In order to advance understanding of the specificity of GH149 enzymes, we herein solved X‐ray crystallographic structures of GH149 enzyme Pro_7066 in the absence of substrate and in complex with laminarihexaose (G6). We have characterized two enzymes from this family, one from the microalga Euglena gracilis, and the other a bacterial enzyme from a metagenomic library, Pro_7066. Both enzymes were shown to have substrate specificity for β‐(1 → 3)‐gluco‐oligosaccharides. The domains present within each subunit can be defined as follows: an N‐terminal β‐sandwich (residues 1‐303, yellow), a helical linker region (residues 304‐341, lilac), an (α/α)6 catalytic domain (residues 342‐1045, green) and a C‐terminal jelly roll domain (residues 1046‐1156, red).

X‐ray crystallography was used to determine the structure of Pro_7066: the substrate‐free structure was solved to 2.05 Å resolution. However, useful data could only be obtained from the G6 co‐crystallization, the structure of which was solved to 2.25 Å resolution. Both structures belong to space group P212121 and contain two subunits per ASU. The two copies of the molecule in the ASU form a biologically relevant homodimer with an interfacial area of ∼4230 Å2 were calculated by jsPISA. The formation of a homodimer in the crystal structure is consistent with the gel filtration analysis, where Pro_7066 was eluted as a dimer. The architecture of the Pro_7066 active site is highly similar to that observed for GH94 enzymes. Bicine (BCN) derived from the crystallization precipitant was bound via hydrogen bonding contacts with R470 and E951, possibly mimicking the interaction of the enzyme active site with the hydroxy groups on C3 and C6 of Glc1P donor. A sulfate molecule was observed (ice blue) occupying a similar position to the phosphate moiety of Glc1P in the PsLBP structure (magenta). Although the RMSD values suggest that these structures are not highly similar (RMSD > 1 Å), the structural elements neighboring the active site are relatively well conserved: (a) the gate (blue) described in PsLBP can be identified in Pro_7066, although in the latter it is part of a disordered loop; (b) the opposing (red) and the adjacent loops (brown), which are present in all of the three structures. In the Pro_7066 structure, Dom 2 (green) is found in proximity to the gate. The average B‐factor of Dom 2 (∼70 Å2) is higher than the average B‐factor of the protein subunit (48 Å2), suggesting Dom 2 is more dynamic compared to the rest of the subunit.

>[2x]MGSSHHHHHHSSGLVPAGSMSQSPNTLANEETTSIDKSITMDMVSMNGEMFYKIANNDAMRPFFMTIVSDSNHWMFVSSNGGLTAGRKNAEYALFPYYTDDKITESADITGSKSIFQIQYNNELIVWEPFSERFTNKFKITRNLYKNYYGNKIIFEEINEDLGLTYRYQWCSSNQFGFVRKSELSNHSKNVYEISLLDGIQNIMPYGVSSDLQSSTSNLVDAYKRSELHPKSGLGIFALSAIIVDKAEPSEALKANIAWSLGLNNPKYLVSSLQLNHFRNGKSISPEDDIKGEKGAYFLNTVMTLEANTQKEWMIIANVNQDHSDIIAITETIQNNKKIAEDINTDIELGTKRLIELNASSDALQLTADNLRDTRHFSNTLFNIMRGGIFDNNYQIEKGDFSNYIKKANKLVFDKIDLNALGEIFSLNDLNEFASKQKDVDFDRLALEYLPLKFSRRHGDPSRPWNKFSINTQSEIDGSKVLDYEGNWRDIFQNWEALAHSFPNFIDSMIHKFLNASTFDGYNPYRVTKEGFDWETIEEDDPWSYIGYWGDHQIIYLLKFLEFIEKHQPGKLHSYFESECFVYAAVPYTIKPYEEILNNPKDTIGYNHEWEKVINERKKSIGADGALLKSNDKSIYHVNFIEKILATVLAKMSNFIPEAGIWLNTQRPEWNDANNALVGNGVSMVTLYYLRRFLKFFDQLLENSTLENIKISNEMVEFYHKVRETLMENQHLLAGSISDTDRKVILDKLGNAAADYRFQIYNSGFWGKKRTHSMQGLKNFTKVSLQFIDHSIKANQRPDKLYHAYNLMSVEKNKEIAISYLSEMLEGQVAVLSSGFLSSKENLAVLDGLKNSALFREDQYSYLLYPNKELPKFLDKNTISKEAVSKSELLSLLVSKSNKQVIEKDSIGEYHFNGEFNNASNLKQALEDLSQQNEYKDLVAKESKTVEAIFEDVFNHKAFTGRSGTFYGYEGLGSIYWHMVSKLQLAVLECCLKAVEEKESEEVIGRLLEHYYEINEGIGVHKSPSLYGAFPTDAYSHTPAGKGAQQPGMTGQVKEDILSRFGELGIFVKNGCLELNPCLLRKDEFLKEAKTFDYVTVNFQHQSLELVEKSLAFTYCQIPIIYKIANQKCIEVFTNDGKSAKAASLILDKQTSQDVFGRTGIINKIEVSILESDLR> MVLADLGRKITSALRSLSNATIINEEVLNAMLKEVCTALLEADVNIKLVKQLRENVKSAIDLEEMASGLNKRKMIQHAVFKELVKLVDPGVKAWTPTKGKQNVIMFVGLQGSGKTTTCSKLAYYYQRKGWKTCLICADTFRAGAFDQLKQNATKARIPFYGSYTEMDPVIIASEGVEKFKNENFEIIIVDTSGRHKQEDSLFEEMLQVANAIQPDNIVYVMDASIGQACEAQAKAFKDKVDVASVIVTKLDGHAKGGGALSAVAATKSPIIFIGTGEHIDDFEPFKTQPFISKLLGMGDIEGLIDKVNELKLDDNEALIEKLKHGQFTLRDMYEQFQNIMKMGPF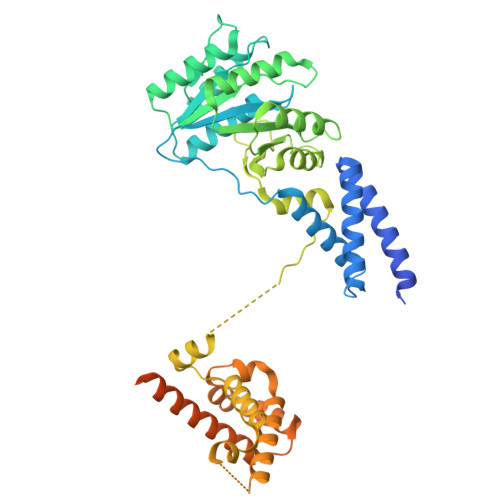SQILGMIPGFGTDFMSKGNEQESMARLKKLMTIMDSMNDQELDSTDGAKVFSKQPGRIQRVARGSGVSTRDVQELLTQYTKFAQMVKKMGGIKGLFKGGDMSKNVSQSQMAKLNQQMAKMMDPRVLHHMGGMAGLQSMMRQFQQGAAGNMKGMMGFNNM>MLQFKKTLLSSIAPVLLSIVLANPVIASDAHHAHKGLNYGSFTKEHVLLTPKGYREWVFIGASVTPNELNDDKAAFPEFHNVYIDPTSWGHWKKTGEFRDGTVIVKELAGVGSKASPSGNGYFPGEFNGIAAMVKDSKRYPERPGNWAFF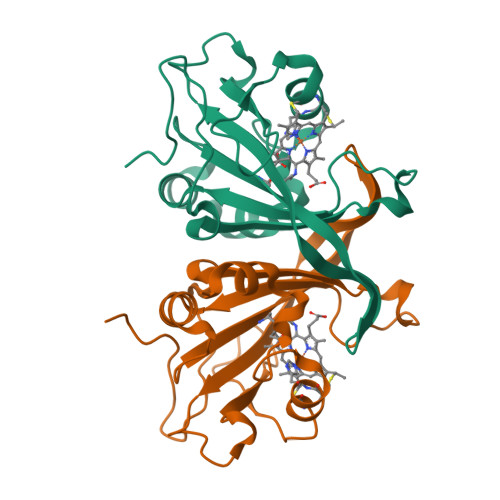GFESYEAKQGIIQTDETCAACHKEHAAHDMVFTQFYPVLRAGKPSK[2x]>EPELTVALILGIFLGTFIA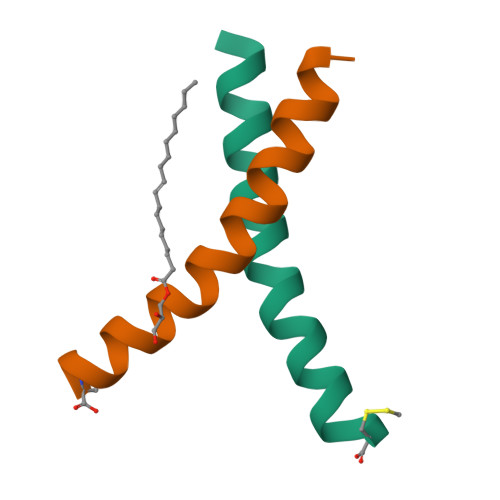FWVVYLLRRLC[6x]> GGCGCUGUGUCGCAAUCUGCGAAGGGCGUCGUCGGCCCAAGCGGUAGUAAGCAGGGAACUCACCUCCAAUGAAACACAUUGUCGUAGCAGUUGACUACUGUUAUGUGAUUGGUAGAGGCUAAGUGACGGUAUUGGCGUAAGCCAAUACCGC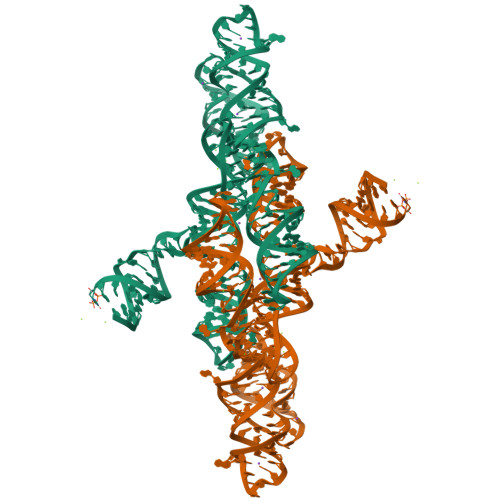AGCACAGCACAAGCCCGCUUGCGAGAUUACAGCGC BuV1 is a member of the Protoparvovirus genus of the Parvoviridae family. Similar to all known parvoviruses, BuV1 assembles into a T = 1 icosahedral capsid. The gross capsid morphology includes pores at the 5-fold vertices, protrusions surrounding the 3-fold axes, a depression region at the 2-fold axes, and a wall separating the depressed regions near the 2- and 5-fold axes. The VPs have an eight-stranded β-barrel motif and an α-helix that form the core of the capsid, which is characteristic of all members of the Parvoviridae.

Additionally, SIA is identified as the terminal glycan receptor for BuV1, and its capsid binding pocket is identified on the 2/5-fold wall. To identify the SIA binding site on the BuV1 capsid, BuV1 VLPs composed of only VP2 were purified. Additional density not attributed to the protein model was clearly visible along the 2-/5-fold wall. Interestingly, only the terminal SIA was able to be fitted into the density in a conformation that leaves the 2′-oxygen exposed to bulk solvent. It is likely that the other two sugar moieties are not visible in the cryo-EM reconstruction due to the flexibility of these moieties in bulk solution, as they are unlikely to interact with the BuV1 capsid, consistent with the observations of the glycan array. The ε-amine of K545 with SIA O10, the backbone carbonyl of Q393 with N5, both the amino nitrogen of Q393 and the ε-amine of K376 to O1B, and the guanidinium moiety of R368 with O1A. Analysis of the binding site by PDBePISA calculated that the sialic acid occludes ~250 Å2 of the capsid surface. However, an overlay of the SIA binding pocket from BuV1 with the structures of BuV2 and BuV3 at pH 7.4 demonstrates that the binding pocket is conserved between these viruses, suggesting that SIA is likely important for cell attachment for these related viruses. The quality of the electron density map allowed for the assignment of most side-chain conformations. However, a surface loop between L495 and N502 exhibited poor density, as previously described, likely due to loop flexibility.

>MPAIRKARGWVPPGYNYLGPFNQDFNKKPTNPSDNAARKHDLEYNKLIKQGHNPYWNYNHADEDFIKETDQATDWGGKFGNFVFRAKRALAPELAPPAKKKTKTKHTEPEYSHKHIKAGTKRGKPFYLFVNLARKKARMTDTQDVSEQQSDQPSVASTNAKAGGGGGGGGSGVGHSTGNYNNRTEFYYHGDEVTIVCHSSRHIHLNMSESEEYKIYDTDRGPRFPTDQTLQGRDTINDSYHAQVETPWFLINPNSWGTWMNPADFQQLTTTCREVTLEHLDQTLDNIVIKTVSKQGSGAEETTQYNNDLTALLQVALDKSNQLPWVADNMYLDSLGYIPWRPCKLKQYSYHVNFWNTIDIISGPQQNQWQQVKKEIRWDDLQFTPIETTTEIDLLRTGDSWTSGPYKFNTKPTQLSYHWQSTRHTGSVHPTDPPNAIGQQGQNIRDINGWQWGDRSDPMSAATRVSNFHIGYSWPEWRIHYGSGGPAINPGAPFSQAPWSTDPQVRLTQGASEKAIFDYNHGDDDPAHRDQWWQNNLPITGQTNWAPKNAHQANLSSNVPSRQEFWTQDYHNTFGPFTAVDDVGIQYPWGAIWTKTPDTTHKPMMSAHAPFICKDGPPGQLLVKLAPNYTENLQTDGLGNNRIVTYATFWWTGKLILKGKLRLPRQFNLYNLPGRPRGTEAKKFLPNEIGHFELPFMPGRCMPNYTM[60x]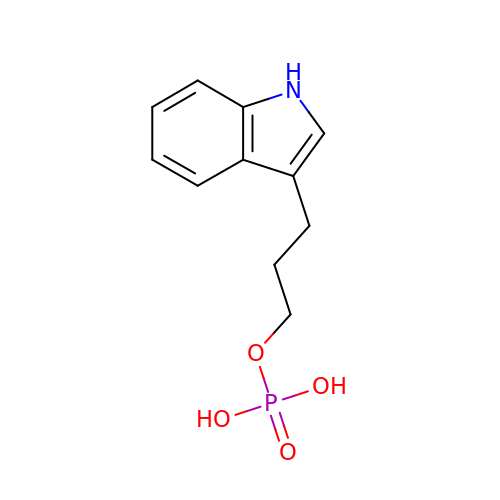INDOLE-3-PROPANOL PHOSPHATE | C11 H14 N O4 P | NKEZSFZOUIIZFL-UHFFFAOYSA-N>[2x]MALRACGLIIFRRCLIPKVDNNAIEFLLLQASDGIHHWTPPKGHVEPGEDDLETALRATQEEAGIEAGQLTIIEGFKRELNYVARNKPKTVIYWLAEVKDYDVEIRLSHEHQAYRWLGLE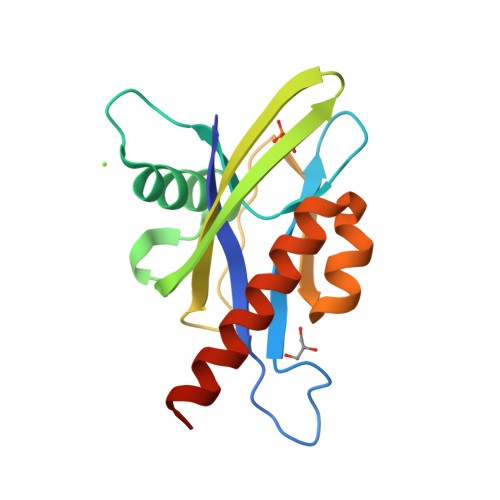EACQLAQFKEMKAALQEGHQFLCSIEALEHHHHHH>[3x]QDKIEALSSKVQQLERSIGLKDLAMADLEQKVLEMEASTYDGV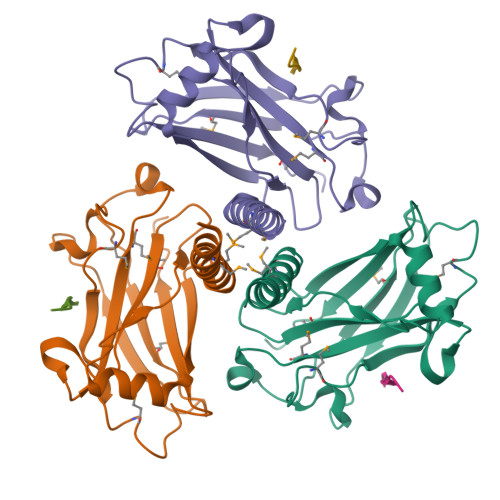FIWKISDFARKRQEAVAGRIPAIFSPAFYTSRYGYKMCLRIYLNGDGTGRGTHLSLFFVVMKGPNDALLRWPFNQKVTLMLLDQNNREHVIDAFRPDVTSSSFQRPVNDMNIASGCPLFCPVSKMEAKNSYVRDDAIFIKAIVDLTGL;>XYPIQET[3x]S-ISOPROPYL-ISOTHIOUREA | C4 H10 N2 S | 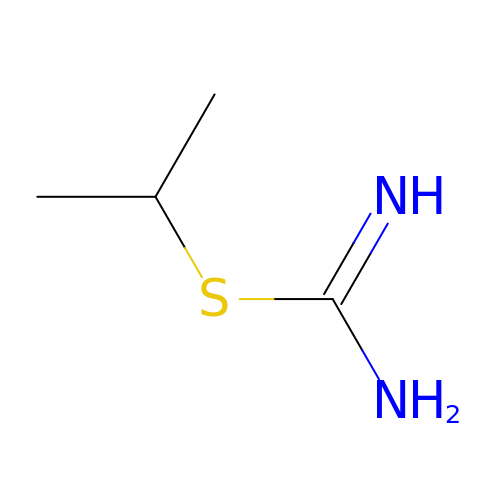XSSNABKEYXKKMK-UHFFFAOYSA-N>KDLGHIVKTIRCLEEEGHIDKSFREDFLTWYSLRATHREVRVVKDFVETFMEDLSSLGQQLVDTFSESI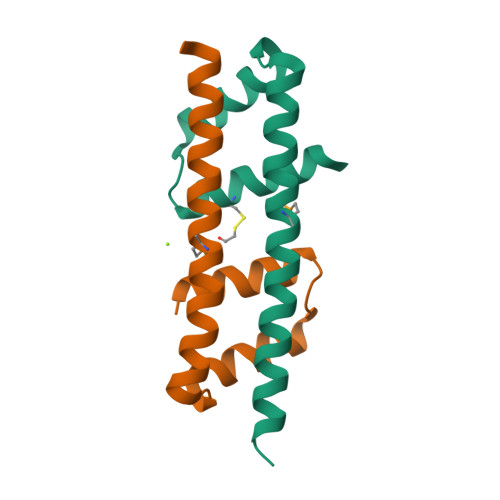LSKK[2x]> HLICQSGDVLSARYEIVDTLGEGAFGKVVECIDHKAGGRHVAVKIVKNVDRYCEAARSEIQVLEHLNTTDPNSTFRCVQMLEWFEHHGHICIVFELLGLSTYDFIKENGFLPF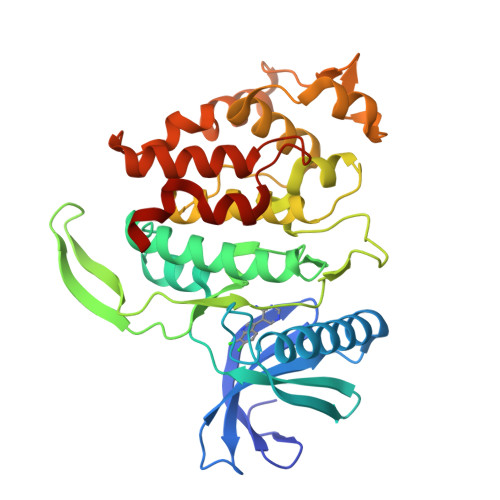RLDHIRKMAYQICKSVNFLHSNKLTHTDLKPENILFVQSDYTEAYNPKIKRDERTLINPDIKVVDFGSATYDDEHHSTLVSTRHYRAPEVILALGWSQPCDVWSIGCILIEYYLGFTVFPTHDSKEHLAMMERILGPLPKHMIQKTRKRKYFHHDRLDWDEHSSAGRYVSRRCKPLKEFMLSQDVEHERLFDLIQKMLEYDPAKRITLREALKHPFFDLLKKSI>[3x]ENLMQVYQQARLSNPELRKSAADRDAAFEKINEARSPLLPQLGLGADYTYSNGYRDANGINSNATSASLQLTQSIFDMSKWRALTLQEKAAGIQDVTYQTDQQTLILNTATAYFNVLNAIDVLSYTQAQKEAIYRQLDQTTQRFNVGLVAITDVQNARAQYDTVLANELTARNNLDNAVEQLRQITGNYYPELAALNVENFKTDKPQPVNALLKEAEKRNLSLLQARLSQDLAREQIRQAQDGHLPTLDLTASTGISDTSYSGSKTRGAAGTQYDDSNMGQNKVGLSFSLPIYQGGMVNSQVKQAQYNFVGASEQLESAHRSVVQTVRSSFNNINASISSINAYKQAVVSAQSSLDAMEAGYSVGTRTIVDVLDATTTLYNAKQELANARYNYLINQLNIKSALGTLNEQDLLALNNALSKPVSTNPENVAPQTPEQNAIADGYAPDSPAPVVQQTSARTTTSNGHNPFRNDYKDDDDK;>MKKRKTVKKRYVIALVIVIAGLITLWRILNAPVPTYQTLIVRPGDLQQSVLATGKLDALRKVDVGAQVSGQLKTLSVAIGDKVKKDQLLGVIDPEQAENQIKEVEAT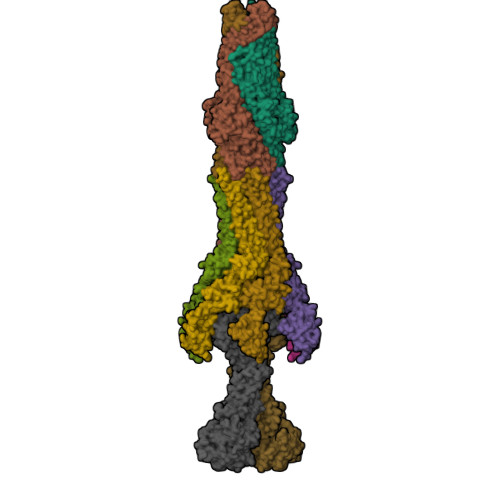LMELRAQRQQAEAELKLARVTYSRQQRLAQTQAVSQQDLDNAATEMAVKQAQIGTIDAQIKRNQASLDTAKTNLDYTRIVAPMAGEVTQITTLQGQTVIAAQQAPNILTLADMSAMLVKAQVSEADVIHLKPGQKAWFTVLGDQLTRYEGQIKDVLPTPEKVNDAIFYYARFEVPNPNGLLRLDMTAQVHIQLTDVKNVLTIPLSALGDPVGDNRYKVKLLRNGETREREVTIGARNDTDVEIVKGLEAGDEVVIGEAKPGAAQ[6x];>[2x]MTPLLELKDIRRSYPAGDEQVEVLKGISLDIYAGEMVAIVGASGSGKSTLMNILGCLDKATSGTYRVAGQDVATLDADALAQLRREHFGFIFQRYHLLSHLTAEQNVEVPAVYAGLERKQRLLRAQELLQRLGLEDRTEYYPAQLSGGQQQRVSIARALMNGGQVILADEPTGALDSHSGEEVMAILHQLRDRGHTVIIVTHDPQVAAQAERVIEIRDGEIVRNPPAIEKVNVTGGTEPVVNTVSGWRQFVSGFNEALTMAWRALAANKMRTLLTMLGIIIGIASVVSIVVVGDAAKQMVLADIRSIGTNTIDVYPGKDFGDDDPQYQQALKYDDLIAIQKQPWVASATPAVSQNLRLRYNNVDVAASANGVSGDYFNVYGMTFSEGNTFNQEQLNGRAQVVVLDSNTRRQLFPHKADVVGEVILVGNMPARVIGVAEEKQSMFGSSKVLRVWLPYSTMSGRVMGQSWLNSITVRVKEGFDSAEAEQQLTRLLSLRHGKKDFFTWNMDGVLKTVEKTTRTLQLFLTLVAVISLVVGGIGVMNIMLVSVTERTREIGIRMAVGARASDVLQQFLIEAVLVCLVGGALGITLSLLIAFTLQLFLPGWEIGFSPLALLLAFLCSTVTGILFGWLPARNAARLDPVDALAREHHHHHH> GSSSGQSNNNSDTCAEFRIKYVGAIEKLKLSEGKGLEGPLDLINYIDVAQ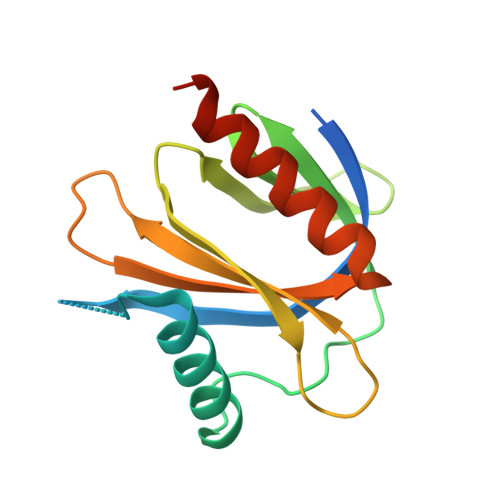QDGKLPFVPPEEEFIMGVSKYGIKVSTSDQYDVLHRHALYLIIRMVCYDDGLGAGKSLLALKTTDASNEEYSLWVYQCNSLEQAQAICKVLSTAFDSVLTSEKP> QPIFLNVLEAIEPGVVCAGHDNNQPDSFAALLSSLNELGERQLVHVVKWAKALPGFRNLHVDDQMAVIQYSWMGLMVFAMGWRSFTNVNSAMLYFAPDLV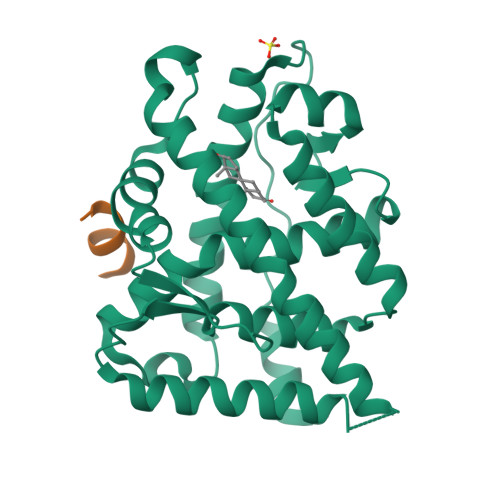FNEYRMHKSRMYSQCVRMRHLSQEFGWLQITPQEFLCMKALLLFSIIPVDGLKNQKFFDELRMNYIKELDRIIACKRKNPTSCSRRFYQLTKLLDSVQPIARELHQFTFDLLIKSHMVSVDFPEMMAEIISVQVPKILSGKVKPIYFHTQ;> KTRYIFDLFYKRKAY α-Galactosidase A (α-Gal A, EC 3.2.1.22) is a lysosomal glycosidase that hydrolyzes the terminal α-linked galactoside present on macromolecules such as globotriaosylceramide (Gb3).1,2 Mutations in the α-galactosidase A gene (GLA) are found in patients with Fabry disease (FD), one of the most common lysosomal storage diseases (LSDs), which is characterized by the progressive accumulation of Gb3 in cells. To unravel the binding mechanism of iminosugars with α-Gal A, N-methylated derivatives 20–24 were synthesized, and we determined the crystal structures of α-Gal A in complex with compounds 4 and 5 at pH 7.2 and 4.5, respectively, and 8, 20, 21, 23, and 24 at pH 7.2 at 1.97 to 2.61 Å resolution.2,32 The structures revealed that these pyrrolidines bind to the catalytic site nearly in the center of the TIM-barrel domain of the enzyme. The bindings are primarily stabilized not only by hydrogen bonds (H-bonds) between the hydroxyl groups of the compounds and the residues D92, D93, L168, D170, E203, R227, and D231 of α-Gal A but also by a salt bridge between the endocyclic amino group (endo-N) of the monobasic compounds (pKa ∼ 7.0) and D170 of the enzyme at pH 7.2.

Previously, the dibasic iminosugar and potent α-Gal A inhibitor 5 having the (2R,3R,4S,5R) configuration pattern demonstrated good chaperoning activity in cells transiently transfected with various mutant α-Gal A.23 Notably, iminosugar 5 exhibited superior pH-dependence in its inhibitory activity compared to its monobasic parent molecule, 4, suggesting that it binds to α-Gal A at pH 7.0 more effectively than 4, leading to better enzyme-stabilizing or chaperoning activity. Surprisingly, in the compound 5-bound structure of α-Gal A, the positively charged exocyclic amino group (exo-N, pKa = 9.1) of 5 forms bifurcated salt bridges (BSBs) with residues E203 and D231 of the enzyme at pH 7.2, where the carboxylic side chains are essentially deprotonated and negatively charged. By contrast, the corresponding C-2 hydroxyl group of 4 forms H-bonds alone to E203 and D231 at pH 7.2. This finding most likely reflects the stronger binding affinity and better protecting effects of 5 toward α-Gal A at pH 7.2 compared to those of 4. In contrast, the titration curves revealed that the endo-N moiety in compound 5 exhibits reduced basicity (pKa = 5.5) compared to that of 4 (pKa = 7.0) due to electrostatic repulsion between the vicinal ammonium cations,34 which implies the formation of an H-bond between endo-N of 5 and D170 at pH 7.0 but a salt bridge at pH 4.5. Given these structural findings, it is conceivable that the pH-dependent protonation states on the amino groups of iminosugars and ionizable residues in the catalytic site of α-Gal A regulate the binding status of the compounds, i.e., the stronger binding of 5 to α-Gal A at pH 7.2 is due to the formation of the BSBs, which are missing at pH 4.5 when the binding is weaker and only H-bonds are formed.

>[2x]LDNGLARTPTMGWLHWERFMCNLDCQEEPDSCISEKLFMEMAELMVSEGWKDAGYEYLCIDDCWMAPQRDSEGRLQADPQRFPHGIRQLANYVHSKGLKLGIYADVGNKTCAGFPGSFGYYDIDAQTFADWGVDLLKFDGCYCDSLENLADGYKHMSLALNRTGRSIVYSCEWPLYMWPFQKPNYTEIRQYCNHWRNFADIDDSWKSIKSILDWTSFNQERIVDVAGPGGWNDPDMLVIGNFGLSWNQQVTQMALWAIMAAPLFMSNDLRHISPQAKALLQDKDVIAINQDPLGKQGYQLRQGDNFEVWERPLSGLAWAVAMINRQEIGGPRSYTIAVASLGKGVACNPACFITQLLPVKRKLGFYEWTSRLRSHINPTGTVLLQLENTMQMSLKDLL>AGITGTWYAQLGDTFIVTAGADGALTGTYEAAVGNAESRYVLTGRYDSAPATDGSGTALGWTVAWKNNYRNAHSATTWSGQYVGGAEARINTQWLLTSGTTEANAWKSTLVGHDTFTKVKPSAAS[3x];> AGITGTWYNQLGSTFIVTAGADGALTGTYESAVGNAESRYVLTGRYDSAPATDGSGTALGWTVAWKNNYRNAHSATTWSGQYVGGAEARINTQWLLTSGTTEANAWKSTLVGHDTFTK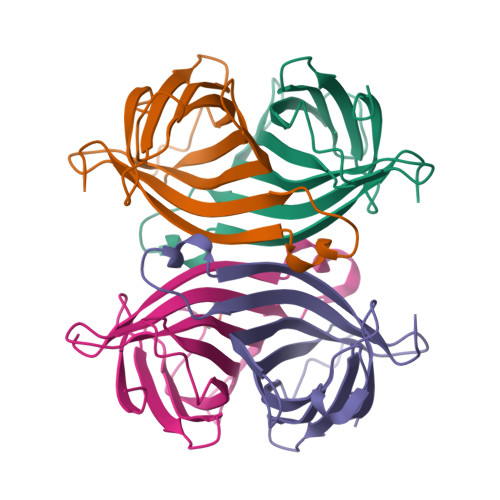VKPSAA> GLSAAQRQVIAATWKDIAGADNGAGVGKKCLIKFLSAHPQMAAVFGFSGASDPGVAALGAKVLAQIGVAVSHLGDEGKMVAQMKAVGVRHKGYGNKHIKAQYFEPL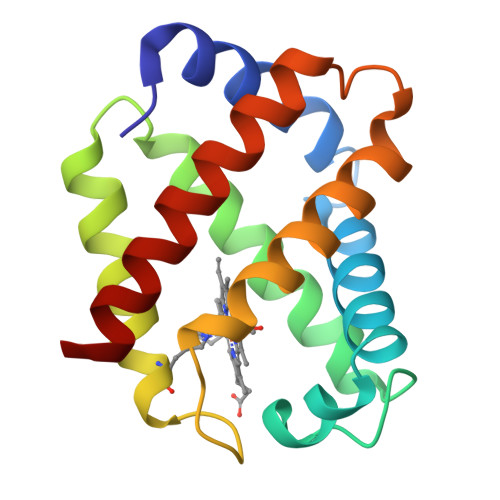GASLLSAMEHRIGGKMNAAAKDAWAAAYADISGALISGLQS> MGSSHHHHHHSSGRENLYFQGMTASIFSGVIPALMTPCRQDRTPDFDALVRKGKELIADGMSAVVYCGSMGDWPLLTDEQRMEGVERLVKAGIPVIVGTGAVNTASAVAHAVHAQKVGAKGLMVIPRVLSRGSVIAAQKAHFKAILSAAPEIPAVIYNSPYYGFATRADLFFALRAEHKNLVGFKEFGGPADMRYAAENITSRDDEVTLMIGVDTAVVHGFVNCGATGAITGIG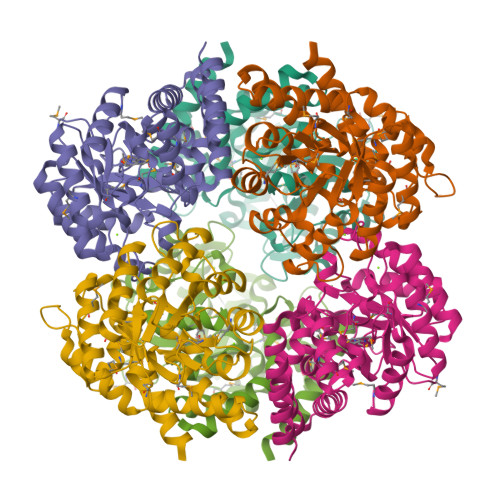NVLPKEVIHLCKLSQAAAKGDADARARALELEQALAVLSSFDEGPDLVLYFKYMMVLKGDKEYTLHFNETDALTDSQRGYVEAQFKLFNSWYADWSKLPGAVQTCKAAGS> GMKEIRIILMGTGNVGLNVLRIIDASNRRRSAFSIKVVGVSDSRSYAS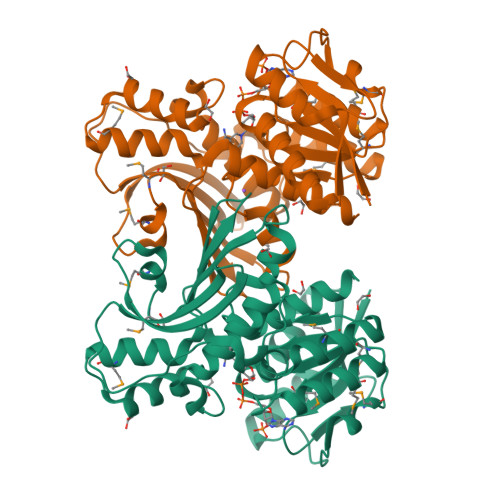GRNLDISSIISNKEKTGRISDRAFSGPEDLMGEAADLLVDCTPASRDGVREYSLYRMAFESGMNVVTANKSGLANKWHDIMDSANQNSKYIRYEATVAGGVPLFSVLDYSILPSKVKRFRGIVSSTINYVIRNMANGRSLRDVVDDAIKKGIAESNPQDDLNGLDAARKSVILVNHIFGTEYTLNDVEYSGVDERSYNANDRLVTEVYVDDRRPVAVSRIISLNKDDFLMSIGMDGLGYQIETDSNGTVNVSDIYDGPYETAGAVVNDILLLSKVQK> MGATKILMDSTHFNEIRSIIRSRSVAWDALARSEELSEIDASTAKALESILVKKNIGDGLSSSNNAHSGFKVNGKTLIPLIHLLSTSDNEDCKKSVQNLIAELLSSDKYGDDTVKFFQEDPKQLEQLFDVSLKGDFQTVLISGFNVVSLLVQNGLHNVKLVEKLLKNNNLINILQNIEQMDTCYV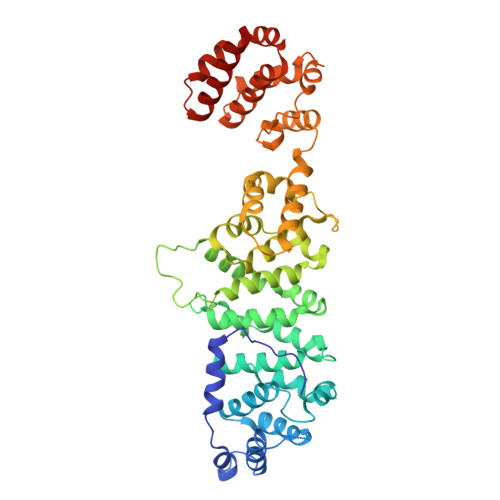CIRLLQELAVIPEYRDVIWLHEKKFMPTLFKILQRATDSQLATRIVATNSNHLGIQLQYHSLLLIWLLTFNPVFANELVQKYLSDFLDLLKLVKITIKEKVSRLCISIILQCCSTRVKQHKKVIKQLLLLGNALPTVQSLSERKYSDEELRQDISNLKEILENEYQELTSFDEYSSELKSGRLEWSPVHKSEKFWRENAVRLNEKNYELLKILTKLLEVSDDPQVLAVAAHDVGEYVRHYPRGKRVIEQLGGKQLVMNHMHHEDQQVRYNALLAVQKLMVHNWE OGA is the unique enzyme responsible for O-GlcNAc hydrolysis from a large number of cytoplasmic and nuclear proteins. Recently, our group and others have independently identified crystallizable constructs of OGA that comprise the catalytic domain and stalk domain, and published the apo form structures and enzyme complexes with active site inhibitors. These reports consistently showed that OGA formed an unusual arm-in-arm homodimer, where the catalytic domain of one monomer covered by the stalk domain of the sister monomer to create a potential substrate-binding cleft. Exploiting our previously reported construct of OGAcryst (residues 60–704 with the unstructured insert residues 401–552 replaced by a glycine–serine (GS) linker), we solved the structures of a mutant OGAcryst-D175N (catalytically impaired but retaining the ability to bind substrate) in apo form and in complex with each of four synthetic glycopeptides.

In the substrate complexes, all the glycopeptides were bound in the OGA substrate-binding cleft. Particularly, the GlcNAc moieties were anchored by the same set of OGA residues in the catalytic pocket, displaying nearly identical binding conformations regardless of the glycosylated residues or the flanking peptide sequences. Consistent with the O-GlcNAc hydrolysis mechanism, the catalytic residue D174 was optimally positioned to make a hydrogen bond with the N-acetyl group of GlcNAc in all the complexed structures. The N175 mutant side chain played an important role in anchoring the glycosylated hydroxyl of serine or threonine and stabilizing the OGA substrate complexes. Intriguingly, the peptide backbone of TAB1 also adopted a V shape, but it was stabilized by an intra-molecular hydrogen bond instead of the interactions with N175. However, the peptide residues of TAB1 oriented dramatically differently in human OGA from those in the bacterial homologs, suggesting that human OGA dimer employs a unique substrate-binding mode. If the peptide bears intra-molecular interactions, it would provide additional stabilization energy for maintaining its ordered binding conformation.

>HFLCGVVEGFYGRPWVMEQRKELFRRLQKWELNTYLYAPKDDYKHRMFWREMYSVEEAEQLMTLISAAREYEIEFIYAISPGLDITFSNPKEVSTLKRKLDQVSQFGCRSFALLFDNIDHNMCAADKEVFSSFAHAQVSITNEIYQYLGEPETFLFCPTEYCGTFCYPNVSQSPYLRTVGEKLLPGIEVLWTGPKVVSKEIPVESIEEVSKIIKRAPVIWDNIHANDYDQKRLFLGPYKGRSTELIPRLKGVLTNPNCEFEANYVAIHTLATWYKSNMNGVRKDVVMTDSEDSTVSIQIKLENEGSDEDIETDVLYSPQMALKLALTEWLQEFGVPHQYSSRGGGGSGGGGSVTLEDLQLLADLFYLPYEHGPKGAQMLREFQWLRANSSVVSVNCKGKDSEKIEEWRSRAAKFEEMCGLVMGMFTRLSNCANRTILYDMYSYVWDIKSIMSMVKSFVQWLGCRSHSSAQFLIGDQEPWAFRGGLAGEFQRLLPIDGANDLFFQ[2x];>[2x]VPYSSAQ>MSNFKVRDPVIQERLDHDYAHHPLVARMNTLDQGNMSQAEYLVQKRHYLVFLIAHHYYEAYLRRMGGIQRRDHLQTLRDQKPRERADRVSAASAYDAGTFTVPSRPGPASGTTPGGQDSLGVSGSSITTLSSGPHSLSPASDILTTLSSTTETAAPAVADARKPPSGKKK[4x];>[2x]MKVQAENAARLGRQVLGLLPPPTHRVSLTRGPEFARGVRDLLSKYAASTRPTVGSLHEALRQAPFRQPTYGDFLVYSQTFSPQEPLGTFLFSFKQEDNGSSMDMLLTPTSLFMLSGMEAAKAPQTHKVAGVWYGSGSGLADFIPNLSELMDTGEFHTLLTPVGPMVQSVHSTFVTKVTSAMKGVGLARDEPRAHVGLTLPCDMLVDLDESCPMVQRREPAGLNVTIYASLVYLRVNQRPSMALTFFQSGKGFAEVVAMIKDHFTDVIRTKYIQLRHELYINRLVFGAVCTLGTVPFDSHPVHQSLNVKGTSLPVLVFANFEAACGPWTVFL;>[4x]MALDKSIVVNLTSRLFADELAALQSKIGSVLPLGDCHRLQNIQALGLGCVCSRETSPDYIQIMQYLSKCTLAVLEEVRPDSLRLTRMDPSDNLQIKNVYAPFFQWDSNTQLAVLPPLFSRKDSTIVLESNGFDIVFPMVVPQQLGHAILQQLLVYHIYSKISAGAPGDVNMAELDLYTTNVSFMGRTYRLDVDNTDPRTALRVLDDLSMYLCILSALVPRGCLRLLTALVRHDRHPLTEVFEGVVPDEVTRIDLDQLSVPDDITRMRVMFSYLQSLSSIFNLGPRLHVYAYSAETLAASCWYSPR;>MEATLEQRPFPYLATEANLLTQIKESAADGLFKSFQLLLGKDAREGSVRFEALLGVYTNVVEFVKFLETALAAACVNTEFKDLRRMIDGKIQFKISMPTIAHGDGRRPNKQRQYIVMKACNKHHIGAEIELAAADIELLFAEKETPLDFTEYAGAIKTITSALQFGMDALERGLVDTVLAVKLRHAPPVFILKTLGDPVYSERGLKKAVKSDMVSMFKAHLIEHSFFLDKAELMTRGKQYVLTMLSDMLAAVCEDTVFKGVSTYTTASGQQVAGVLETTDSVMRRLMNLLGQVESAMSGPAAYASYVVRGANLVTAVSYGRAMRNFEQFMARIVDHPNALPSVEGDKAALADGHDEIQRTRIAASLVKIGDKFVAIESLQRMYNETQFPCPLNRRIQYTYFFPVGLHLPVPRYSTSVSVRGVESPAIQSTETWVVNKNNVPLCFGYQNALKSICHPRMHNPTQSAQALNQAFPDPDGGHGYGLRYEQTPNMNLFRTFHQYYMGKNVAFVPDVAQKALVTTEDLLHPTSHRLLRLEVHPFFDFFVHPCPGARGSYRATHRTMVGNIPQPLAPREFQESRGAQFDAVTNMTHVIDQLTIDVIQETAFDPAYPLFCYVIEAMIHGQEEKFVMNMPLIALVIQTYWVNSGKLAFVNSYHMVRFICTHMGNGSIPKEAHGHYRKILGELIALEQALLKLAGHETVGRTPITHLVSALLDPHLLPPFAYHDVFTDLMQKSSRQPIIKIGDQNYDNPQNRATFINLRGRMEDLVNNLVNIYQTRVNEDHDERHVLDVAPLDENDYNPVLEKLFYYVLMPVCSNGHMCGMGVDYQNVALTLTYNGPVFADVVNAQDDILLHLENGTLKDILQAGDIRPTVDMIRVLCTSFLTCPFVTQAARVITKRDPAQSFATHEYGKDVAQTVLVNGFGAFAVADRSREAAETMFYPVPFNKLYADPLVAATLHPLLANYVTRLPNQRNAVVFNVPSNLMAEYEEWHKSPVAAYAASCQATPGAISAMVSMHQKLSAPSFICQAKHRMHPGFAMTVVRTDEVLAEHILYCSRASTSMFVGLPSVVRREVRSDAVTFEITHEIASLHTALGYSSVIAPAHVAAITTDMGVHCQDLFMIFPGDAYQDRQLHDYIKMKAGVQTGPPGNRMDHVGYAAGVPRCENLPGLSHGQLATCEIIPTPVTSDVAYFQTPSNPRGRAACVVSCDAYSNESAERLLYDHSIPDPAYECRSTNNPWASQRGSLGDVLYNITFRQTALPGMYSPCRQFFHKEDIMRYNRGLYTLVNEYSARLAGAPATSTTDLQYVVVNGTDVFLDQPCHMLQEAYPTLAASHRVMLDEYMSNKQTHAPVHMGQYLIEEVAPMKRLLKLGNKVVY[4x];> MDAHAINERYVGPRCHRLAHVVLPRTFLLHHAIPLEPEIIFSTYTRFSRSPGSSRRLVVCGKRVLPGEENQLASSPSGLALSLPLFSHDGNFHPFDISVLRISCPGSNLSLTVRFLYLSLVVAMGAGRNNARSPTVDGVSPPEGAVAHPLEELQRLARATPDPAPTRGPLQVLTGLLRAGSDGDRATHHMALEAPGTVRGESLDPPVSQKGPARTRHRPPPVRLSFNPVNADVPATWRDATNVYSGAPYYVCVYERGGRQEDDWLPIPLSFPEEPVPPPPSLVFMDDLFINTKQCDFVDTLEAACRTQGYTLRQRVPVAIPRDAEIADAVKSHFLEACLVLRGLASEASAWIRAATSPPLGRHACWMDVLGLWESRPHTLGLELRGVNCGGTDGDWLEILKQPDVQKTVSGSLVACVIVTPALEAWLVLPGGFAIKGRYRASKEDLVFIRGRYG;>[2x]MLTSERSYLRYPKNRRWTEAGRFWAPHPENVLFIHKPTMEETRRVALGLRSQLVRNRERKTKAHLLSLELDRLVQVHDSRVRVINADIDAVKQMIGNMTWSDNIDMPQSRSHEPPLVTSPPQASHRNFTVAIVPGDPHFSVDRDLRGELMPTLYMNQNQWLPSFGPWFISLTDNAMQRRVFPKELKGTVNFQNSTSLKLISHTLTTVASTTADFFADARHLTDTQAALCLVNAYFCQKTSRQLPATPDDLLADLPQKLDLLITQLKQESGPGDFSFTYSNPQERASLAPLNKESRYPTAFFQRHKLHAMMAKAGLFPHNKGTGAPGTAPAMDLVFAITSAMFGSDIPPFSAYQWNLRAGIVALEVFILAYGLLEFGQVARGHPNRRLNLVSLLGPKFQPGALPDPNAPMLKRGQLFSFISEHYIIPTLQANPNAPVSFIFPGIILAALEARSTVSHKQPGPFVNLTGSRFNEIFEILNQQLTFRDPLALLQARTALRLATEEGLDVLLSHPSPPTLLQEIIKSQFGGGDDYDRAYFMVLGCLPVVLAVV;>MAAQPLYMEGMASTHQANCIFGEHAGSQCLSNCVMYLASSYYNSETPLVDRASLDDVLEQGMRLDLLLRKSGMLGFRQYAQLHHIPGFLRTDDWATKIFQSPEFYGLIGQDAAIREPFIESLRSVLSRNYAGTVQYLIIICQSKAGAIVVKDKTYYMFDPHCIPNIPNSPAHVIKTNDVGVLLPYIATHDTEYTGCFLYFIPHDYISPEHYIANHYRTIVFEELHGPRMDISRGVESCSITEITSPSVSPAPSEAPLRRDSTQSQDETRPRRPRVVIPPYDPTDRPRPPHQDRPPEQAAGYGGNKGRGGNKGRGGKTGRGGNEGRGGHQPPDEHQPPHITAEHMDQSDGQGADGDMDSTPANGETSVTETPGPEPNPPARPDREPPPTPPATPGATALLSDLTATRGQKRKFSSLKESYPIDSPPSDDDDVSQPSQQTAPDTEDIWIDDPLTPLYPLTDTPSFDITADVTPDNTHPEKAADGDFTNKTTSTDADRYASASQESLGTLVSPYDFTNLDTLLAELGRLGTAQPIPVIVDRLTSRPFREASALQAMDRILTHVVLEYGLVSGYSTAAPSKCTHVLQFFILWGEKLGIPTEDAKTLLESALEIPAMCEIVQQGRLKEPTFSRHIISKLNPCLESLHATSRQDFKSLIQAFNAEGIRIASRERETSMAELIETITARLKPNFNIVCARQDAQTIQDGVGLLRAEVNKRNAQIAQEAAYFENIITALSTFQPPPQSQQTFEVLPDLKLRTLVEHLTLVEAQVTTQTVESLQAYLQSAATAEHHLTNVPNVHSILSNISNTLKVIDYVIPKFIINTDTLAPYKQQFSYLGGELASMFSLDWPHAPAEAVEPLPVLTSLRGKIAEALTRQENKNAVDQILTDAEGLLKNITDPNGAHFHAQAVSIPVLENYVHNAGVLLKGEKSERFSRLKTAIQNLVSSESFITVTLHSTNLGNLVTNVPKLGEAFTGGPHLLTSPSVRQSLSTLCTTLLRDALDALEKKDPALLGEGTTLALETLLGYGSVQDYKETVQIISSLVGIQKLVRDQGADKWATAVTRLTDLKSTLATTAIETATKRKLYRLIQRDLKEAQKHETNRAMEEWKQKVLALDNASPERVATLLQQAPTAKAREFAEKHFKILLPVPADAPVQASPTPMEYSASPLPDPKDIDRATSIHGEQAWKKIQQAFKDFNFAVLRPADWDALAAEYQRRGSPLPAAVGPALSGFLETILGTLNDIYMDKLRSFLPDAQPFQAPPFDWLTPYQDQVSFFLRTIGLPLVRALADKISVQALRLSHALQSGDLQQATVGTPLELPATEYARIASNMKSVFNDHGLQVRSEVADYVEAQRADAHTPHVPRPKIQAPKTLIPHPDAIVADGLPAFLKTSLLQQEAKLLALQRADFESLESDMRAAEAQRKASREETQRKMAHAITQLLQQAPSAISGRPLSLQDPVGFLEGIIYDKVLERESYETGLEGLSWLEQTIKSITVYAPVEEKQRMHVLLDEVKKQRANTETALELEAAATHGDDARLLQRAVDELSPLRVKGGKAAVESWRQKIQTLKSLVQEAEQAGLLLATIDTVAGQAQETISPSTLQGLYQQGQEAMAAIKRFRDSPQLAGLQEKLAELQQYVKYKKQYLEHFEATQSVVFTAFPLTQEVTIPALHYAGPFDNLERLSRYLHIGQTQPAPGQWLLTLPTFDPTRPACVPAGGHEPPLHRQVVFSSFLEAQIRLALSVAGPVPGRGLPGTPQIRRGVEAAACFLHQWDEISRLLPEVLDTFFHNAPLPAESSSNAFLAMCVLTHLVYLAGRAVLGPREPEHAAPDAYPREVALAPRDLTYLLLAMWPSWISAILKQPSHAEAAHACLVTLPTMLKAVPYLTLEASAGPLPADMRHFATPEARLFFPARWHHVNVQEKLWLRNDFMSLCHRSPGRARIAVLVWAVTCLDPEVIRQLWSTLRPLTADESDTASGLLRVLVEMEFGPPPKTPRREAVAPGATLPPYPYGLATGERLVGQAQERSGGAGKMPVSGFEIVLGALLFRAPLRIFSTASTHRISDFEGGFQILTPLLDCCPDREPFASLAAAPRRTVPLGDPCANIHTPEEIQIFARQAAWLQYTFANYQIPSTDNPIPIVVLNANNNLENSYIPRDRKADPLRPFYVVPLKPQGRWPEIMTTATTPCRLPTSPEEAGSQFARLLQSQVSATWSDIFSRVPERLAPNATQKSSQTMSEIHEVAATPPLTITPNKPTGTPHVSPEADPITERKRGQQPKIVADNMPSRILPSLPTPKPREPRITLPHALPVISPPAHRPSPIPHLPAPQVTEPKGVLQSKRGTLVLRPAAVIDPRKPVSAPITRYERTALQPPRTEGEGRRPPDTQPVTLTFRLPPTAPTP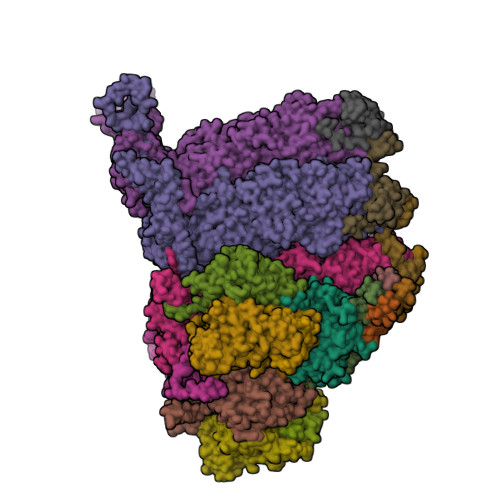ATAALETKTTPPSTPPHAIDISPPQTPPMSTSPHARDTSPPAEKRAAPVIRVMAPTQPSGEARVKRVEIEQGLSTRNEAPPLERSNHAVPAVTPRRTVAREIRIPPEIKAGWDTAPDIPLPHSSPESSPPTSPQPIRVDDKSPLPNLVERYARGFLDTPSVEVMSLENQDIAVDPGLLTRRIPSVVPMPHPIMWSPIVPISLQNTDIDTAKITLISFIRRIKQKVAALSASLAETVDRIKKWYL[2x]>GATESGKRMDCPALPPGWKKEEVIRKSGLSAGKSDVYYFSPSGKKFRSKPQLARYLGNTVDLSSFDFRTGKMMPSKLQK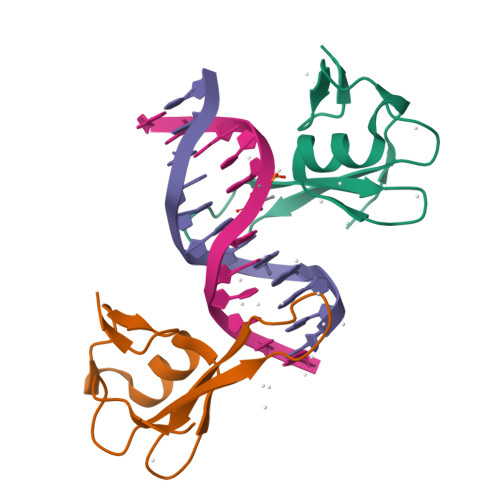[4x]>MTRIAIALAQDFADWEPALLAAAARSYLGVEIVHATPDGMPVTSMGGLKVTPDTSYDALDPVDIDALVIPGGLSWEKGTAADLGGLVKRFRDRDRLVAGICAAASALGGTGVLNDVAHTGNALASHKAYPAYRGEAHYRDQPRAVSDGGVVTAAGSAPVSFAVEILKSLGLFGP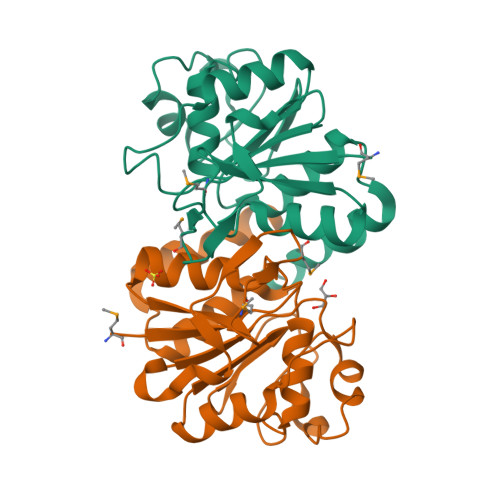EAEAELQIFAAEHR[3x]>MANPYERGPDPTESSIEAVRGPFAVAQTTVSRLQADGFGGGTIYYPTDTSQGTFGAVAISPGFTAGQESIAWL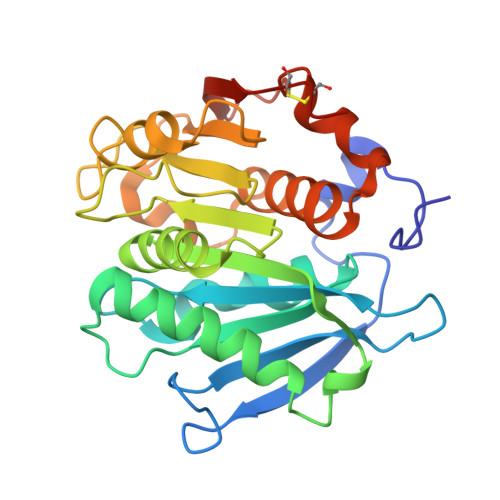GPRIASQGFVVITIDTITRLDQPDSRGRQLQAALDHLRTNSVVRNRIDPNRMAVMGHSMGGGGALSAAANNTSLEAAIPLQGWHTRKNWSSVRTPTLVVGAELDTIAPVSSHSEAFYNSLPSDLDKAYMELRGASHTVSNTPDTTTAKYSIAWLKRFVDKDLRYEQFLCPAPDDFAISEYRSTCPFLEHHHHHH[2x]> RRNLKG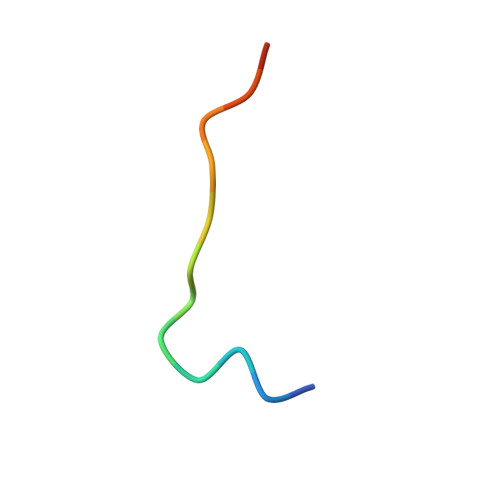LNLNLHPD> MGEKRKTRQAEVNIGMVGHVDHGKTTLTKALTGVWTDTHSEELRRGITIKIGFADAEIRRCSNCGRYSTSPICPYCGHETEFIRRVSFIDSPGHEALMTTMLAGASLMDGAILVIAANEPCPRPQTREHLMALQIIGQKN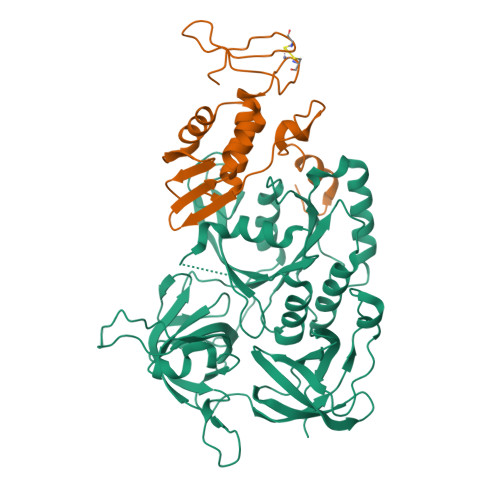IIIAQNKIELVDKEKALENYRQIKEFIKGTVAENAPIIPISALHGANIDVLVKAIEEFIPTPKRDSNKPPKMLVLRSFDVNKPGTPPEKLVGGVLDGSIVQGKLKVGDEIEIRPGVPYEEHGRIKYEPITTEIVSLQAGGQFVEEAYPGGLVGIGTKLDPYLTKGDLMAGNVVGKPGKLPPVWTDLRLEVHLLERVVGTEQELNVEPIKRKEVLLLNVGTARTMGLVTALGKDEIELKLQIPVCAEPGERVAISRQIGSRWRLIGYGIIKELEHHHHHH;> MEIDYYDYEKLLEKAYQELPENVKHHKSRFEVPGALVTIEGNKTIIENFKDIADALNRDPQHLLKFLLREIATAGTLEGRRVVLQGRFTPYLIANKLKKYIKEYVICPVCGSPDTKIIKRDRFHFLKCEACGAETPIQHLLEHHHHHH> APCEPESLEINKYFVVIIYALVFLLSLLGNSLVMLVILYSRVGRSVTDVYLLNLALADLLFALTLPIWAASKVNGWIFGTFLCKVVSLLKEVNFYSGIWLLACISVDRYLAIVHATRTLTQKRYLVKFICLSIWGLSLLLALPVLLFRRTVYSSNVSPACYEDMGNNTANWRMLLRILPQSFGFIVPLLIMLFCYGFTLRTLFKAGIDCSFWNESYLTGSRDERKKSLLSKFGMDEGVTFMFIGRFDRGQKGVDVLLKAIEILSSKKEFQEMRFIIIGKGDPELEGWARSLEEKHGNVKVITEMLSREFVRELYGSVDFVIIPSYFEPFGLVALEAMCLGAIPIASAVGGLRDIITNETGILVKAGDPGELANAILKALELSRSDLSKFRENCKKRAMSFSGQKHREMRVIFAVVLIFLLCWLPYNLVL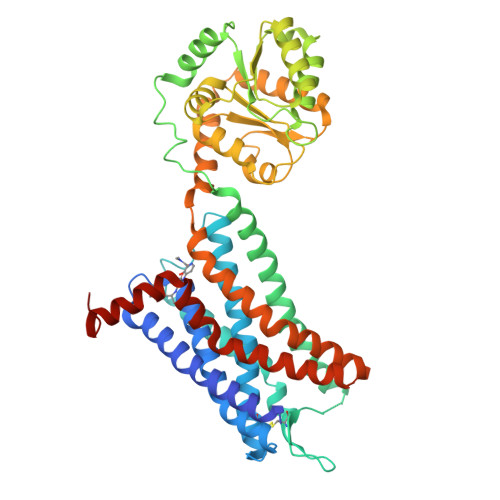LADTLMRTQVIQETCERRNHIDRALDATEILAILHSCLNPLIYAFIGQKFRHGLLKILAIHGLISKDSLPKDS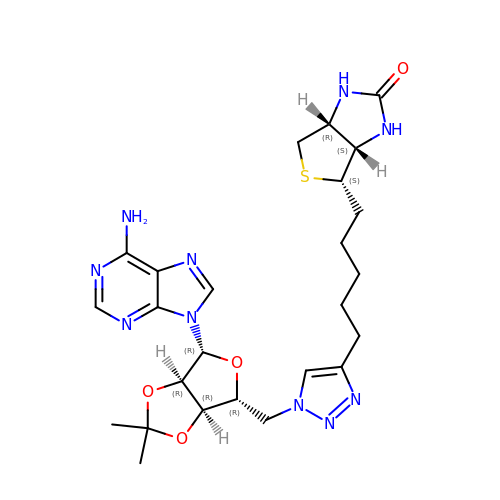5'-deoxy-2',3'-O-(1-methylethylidene)-5'-(4-{5-[(3aS,4S,6aR)-2-oxohexahydro-1H-thieno[3,4-d]imidazol-4-yl]pentyl}-1H-1,2,3-triazol-1-yl)adenosine | C25 H34 N10 O4 S | JOAMEQGLLLPUCO-SGEVEQOLSA-N> FSNECLGTIGPVTPLDASDFALDIRMPGVTPKESDTYFCMSMRLPVDEEAFVIDFKPRASMDTVHHMLLFGCNMPSSTGSYWFCDEGTCTDKANILYAWARNAPPTRLPKGVGFRVGGETGSKYFVLQVHYGDISAFRDNHKDCSGVSVHLTRVPQPLIAGMYLMMSVDTVIPPGEKVVNADISCQYKMYPMHVFAYRVHTHHLGKVVSG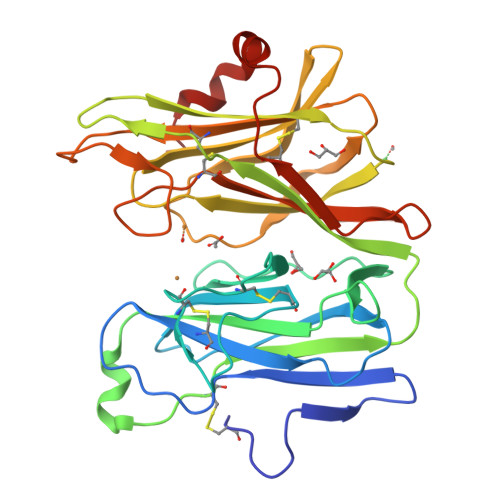YRVRNGQWTLIGRQNPQLPQAFYPVEHPVDVTFGDILAARCVFTGEGRTEATHIGGTSSDEMCNLYIMYYMEAKYALSFMTCTKNVAPDMFRTIPAEANIPIPV>[2x]MSTFIIRLLIFSLLCGSFSIHAEEQNGMKLERVVIVSRHGVRAPTKFTPIMKNVTPDQWPQWDVPLGWLTPRGGELVSELGQYQRLWFTSKGLLNNQTCPSPGQVAVIADTDQRTRKTGEAFLAGLAPKCQIQVHYQKDEEKNDPLFNPVKMGKCSFNTLQVC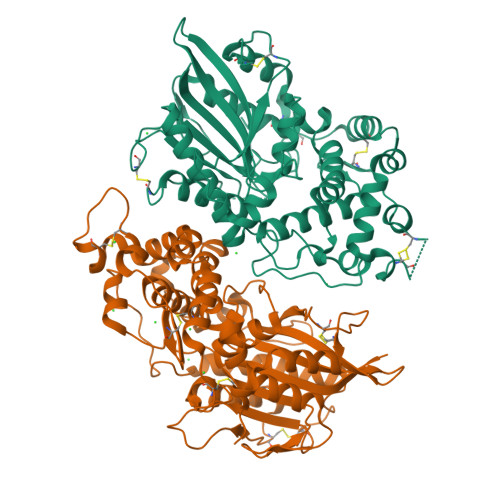NAILERAGGNIELYTQRYQSSFRTLENVLNFSQSETCKTTEKSTKCTLPEALPSELKCTPDNVSLPGAWSLSSTLTEIFLLQEAQGMPQVAWGRITGEKEWRDLLSLHNAQFDLLQRTPEVARSRATPLLDMIDTALLTNGTTENRYGIKLPVSLLFIAGHDTNLANLSGALDLNWSLPGQPDNTPPGGELVFEKWKRTSDNTDWVQVSFVYQTLRDMRDIQPLSLEKPAGKVDLKLIACEEKNSQGMCSLKSFSRLIKEIRVPECAVTE> GPDWVVA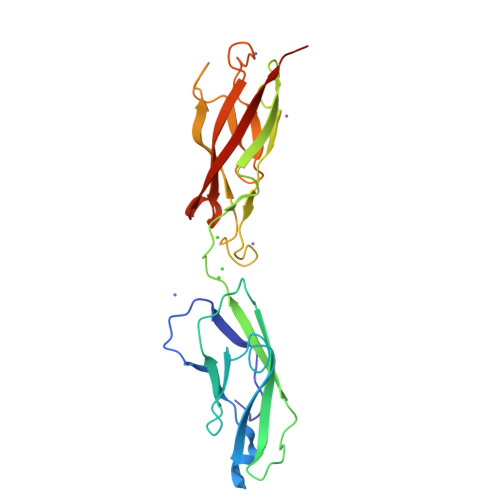PISVPENGKGPFPQRLNQLKSNKDRDTKIFYSITGPGADSPPEGVFAVEKETGWLLLNKPLDREEIAKYELFGHAVSENGASVEDPMNISIIVTDQNDHKPKFTQDTFRGSVLEGVLPGTSVMQVTATDEDDAIYTYNGVVAYSIHSQEPKDPHDLMFTIHRSTGTISVISSGLDREKVPEYTLTIQATDMDGDGSTTTAVAVVEILDANDN> TPEVGELIEKVRKAHQETFPALCQLGKYTTNNSSEQRVSLDIDLWDKFSELSTKCIIKTVEFAKQLPGFTTLTIADQIT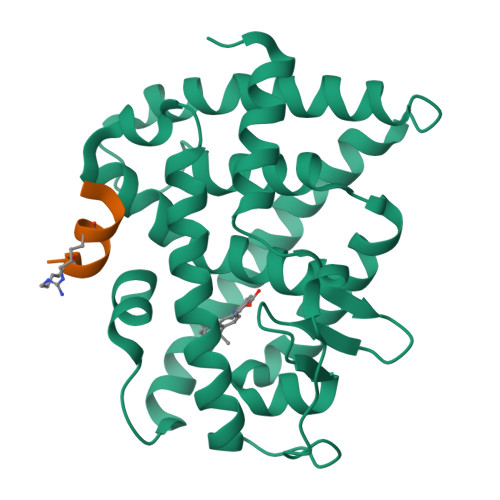LLKAACLDILILRICTRYTPEQDTMTFSDGLTLNRTQMHNAGFGPLTDLVFAFANQLLPLEMDDAETGLLSAICLICGDRQDLEQPDRVDMLQEPLLEALKVYVRKRRPSRPHMFPKMLMKITDLRSISAKGAERVITLKMEIPGSMPPLIQEMLE;> XAHLILHRLLA2-[4-(2,4-DICHLOROPHENOXY)PHENOXY]PROPANOIC ACID 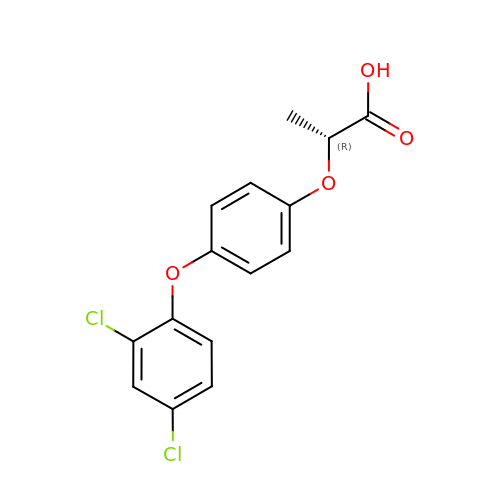| C15 H12 Cl2 O4 | OOLBCHYXZDXLDS-SECBINFHSA-N>ATTPSANQNWRLLRDESAQLRIADVLQRKEQFRPLAKRSFIFPASPQAVWLQVQLPAQKVPSWLWIFAPRVQYLDYYLVQDGQLVRDQHTGESRPFQERPLPSRSYLFSLPVDGKPMTLYVRMTSNHPLMAWFDQ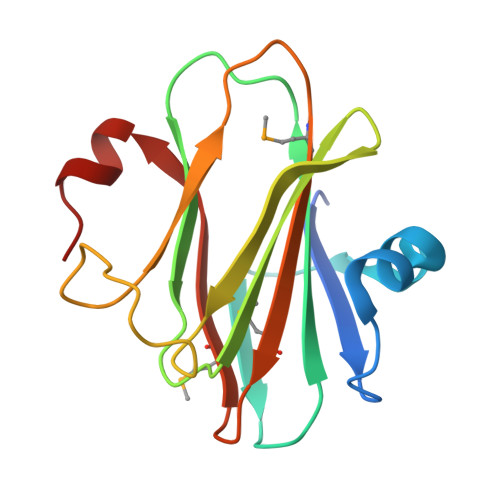IDEAGLVGLE[2x]>PLGSKDNRLLYPKTKIDWGPGENHICLKTPFKNFYVIELFHQAPTFDKTIPLFISDINNSPNLYGIYNYIADHLRHVVLVNNYPVNQINIFGKIVYEQYKEKEFNGVEESYVILVISDFIGIDSKIRVRLSQEQFKEVGLTLDKKNYGKIVELEGEIYNWYDSINVSKKPDRELKVSKITVLSHRPDGLHFEFEQWKKRMEFRKNNLVEPWVFIPTPQRE[2x];>SSKIILIPSNIPQEFPEASISNPERLRILAQVKDFIPHESTIVIDKVPTITSEQSTYINICIFNLLEACSSRVLVPGTLVNIDAFYDGESINPVDI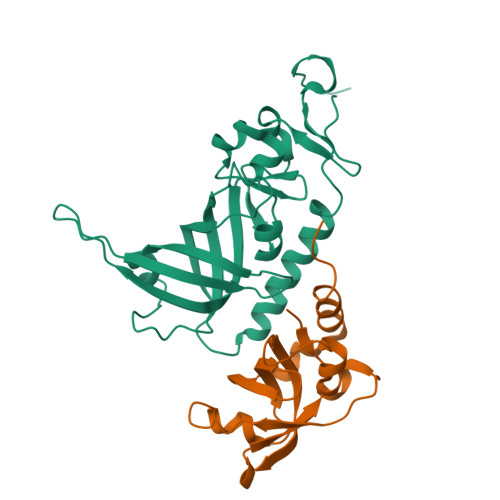YEVNGANFTMENIQLIDEMNNSIGKFN[2x]(3Z)-N-[(1S)-2-hydroxy-1-phenylethyl]-3-[(1H-imidazol-2-yl)(phenyl)methylidene]-2-oxo-2,3-dihydro-1H-indole-5-carboxamide | C27 H22 N4 O3 | 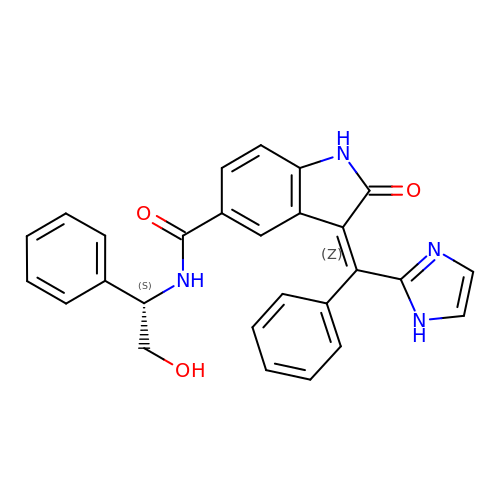ZYTOTYXABPGGHD-PDWGEAQMSA-N> MTDRPFILQVPPTQQRGPQNIAEFVARINPDAFRVLNEAELRRKVEEEKNGVGQDEDVDMESSPSDNEGEPADAKDIITAKHEMLRVIDQTRQTTLYALDFVSLLLSKENPGQAVTTFSPGLRELVGIGTLGATMLDAPTPLTQSRIPDNKLVTIGKRLMDLNKAADTAL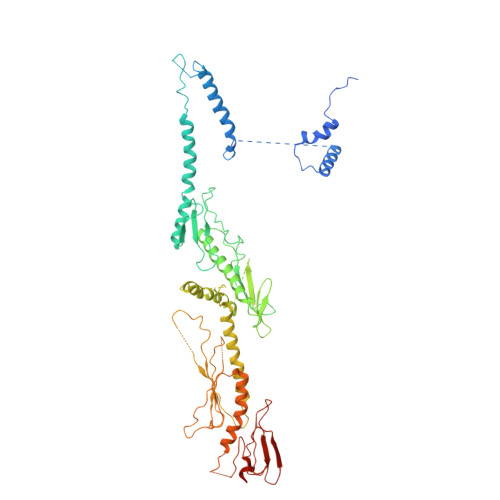AASKRLQKEIAAETKYWSEVLAVRNDGWQTSRMPREPQTMGVKFGFNNAAPEFKAVSIAPMRRADNGSVLLDRSSIGHKSQRIQVRILEDGRIVGRSSLPSPVSADAPLQDRVKEMRDTIFAQELWHEINREARTLLNQGVHLEPSSITYTMDASTTVSIRLATLGEEEEGLDEQQEGPQDVMAESLNIALSLLLSHAHRMNELRRSEPGINKGPPRTYPILLPLISYHKYNQSIQTCLQTLSAHISVLRSASVDSSMTVKEPLLSSPPGAPAATSLYTILTRPPAVQFDITITPDSRIRILLKPTQLTGAAFSICCLPALHPGAQNPLATTCPPSTDDYDSLTQVVSYLQAAIPRALAAHYEAVLVVEATVNGGMLGDLPPSPSRWMPLIDGKGIVDPETMRFGIRFSFGRNPAKGGQLELGAQTDYVDGSRKRVRRNWIWPGAQSSLDSVAKHVLARGPPEE> TVAAYNLTWKSTNF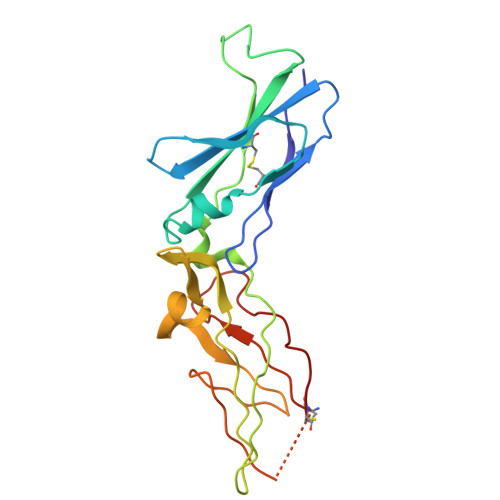KTILEWEPKPVNQVYTVQISTKSGDWKSKCFYTTDTECDLTDEIVKDVKQTYLARVFSYPAGNVESTGSAGEPLYENSPEFTPYLETNLGQPTIQSFEQVGTKVNVTVEDERTLVRRNNTFLSLRDVFGKDLIYTLYYWKSSSSGKKTAKTNTNEFLIDVDKGENYCFSVQAVIPSRTVNRKSTDSPVEC> MVIYGTGIDLTELSRIEAILAKGLRLPEKILTPAELAVFSRYPVKRQIEFMAGRFSAKEAYSKAYGTGIGAAVGFQDIEILDNAQGKPEVTRH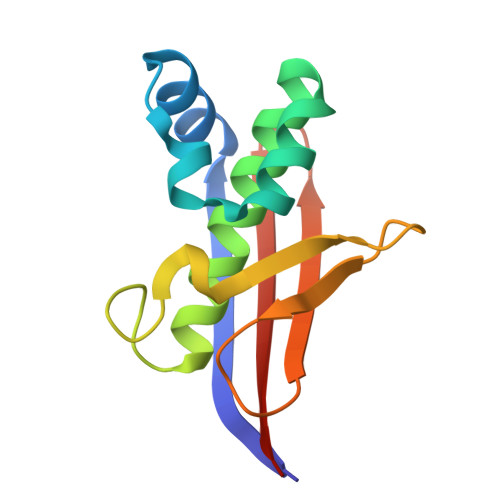PFDGPAWISISHTDTLVMTQVILERGNL>MATNQQLSIALRIQADLAEAQNALRQLTGNLQQVDRGAVQTRSELSAMGGQLDSLRAQVLGFVGAWASLSALGGLVTMVDQYGQMADRIQMVTSSTAEYEQVQARLLETASRTYRPLAEAQELYIRTADSLKSLRYTTEQALDITDSFSFLLVTNAASADRAASAIDAYSKSIQTGKVSSDAWQSIMAAMPSLVNALAESTGKSTEEIRKLGIEGSLSLRDLNEGLRKTVAANREAADNMGTSVQDALVSLNNALSAYLGELNRTYDITGSVSSALNVLAENMEVIVKLFGVAAVAGLTRYVASLTLATQAKLAAVLAARAQAAEELRTAQAQVASTAAAAANARAQAGLTVSHTQAAAAEAAHTAATQRLAAAQLAAGAAMRGMLAVIGGPAGIAMLVAGAAASFFLFRDSAQAVKSSLDDLSEPLDQVVERMGKLSEIEQDRELTRLSEQIDGLRQTAVEAAREMREVASTALYGARLDRIPSAEAQQALQPLIDASADAARGVEVDWKSVMDTLAASGAVPDSLKRKLLDMAAGQAEAGRTATELGQRHAELKARLEGSTAAINENSDALSKGSDKAAEYIQSLRLAIADLEDPSVLGKAGRRLQQFGADLNAEQSAEILRLETLKANTEKAAQAREDARRKAESSARQQASTAEQLAKSQEGYVAGLEKQARTLGLTSAEVRAYELAEKGLTGALHARAAAALAALAADEKKRQADANARTNAGLEAEYLRATGRTVDAGLLEIRTKFDAMRRDFEKAGNDAGLAWIDKLIPVAEAKVRLDDVKQQMDDLLADQQRAESSVNVQQDAGVINEMDARQRILDIHRATYEKLQQIRPILEQMARQPGEVGRAAAESLAQLDAEAARLQQTTTLLETTLRDGLTTGFTDAIKGLASGTMDLRDAITSLGEAVLNALVNMAAQNLAQSLSSGIMGLFGGGQQDTSMTTGAAAVTASAGALSTAGASLLTGAAAIQAAAASLAAANGVQGLGAAAGGAGAAGAAAGGGSWLSSIAGIFGFASGGHIKGPGTGTSDSIPILASNDEFMTRAAVVRQPGALAFLEQFNRYGMAALAGWANPVRHATGGQIGTPAPNLPAPVRAGANLPEPSKNFSTSVANSIYLHAVQDTDQMAADMWAGKGGEHFLVWLNKNRQAVKQII[3x];>MATFPGFQVPKPVEGIVAGITPNIDALELNQDISLAAVAASTWGGAYGAHQPVEVIHSTYQAVHQSALEENYYNRLWLIPTAMELGNVVSTQIRPASVWNAYFSPRTLTAIDREAADGITLSGQASPPLGFAALEERTWTVSIGTDGPPVVNARIVWRLQGEPNLVLVITGNRIIAWTFAPDWGDSIVERLSASTNILQSESAVTQRRAMRLAPRREFDANMYAVDRERQLLDMTLFGWGARIWALPIWPDIQLLHQPLAAGSLGIPCDTAGLDFRDGGLAMLRGEDAFTYEVVEVKTVTASGLDLVRPVQAAWGTGSRLYPVRTAQLTEQPTLTRLTDTAQSARVSFLVMEPSAWPELMPATTYRGRPVLEQRPDESEDLTSSYQRLLSTLDNGSAIPRVTDVAGMALPVIGHRWIGMGRAERSAFRSLVYALRGQQKPLWVPTHADDLTLVATVSQLSTALDVRNIGYARFANGRPGRRDIRIELYDGTVYHRRILTSTELDADTERVAIDAALGRLVEPTDVARICFMALCSAASDVVEIEHVTDSEGVATAALTFKGVRDDEF[3x];>MTLYMGPNTGLLINGLPGEGHYSDLIRMWRWDDFLRQPVVKGRVATLPTTGQAEGDTYIFTGSGSNQNRLARWWATGATTAIWEYMPPRLGWRVQVANETTPSGQVKTYEYSGTAWVELVGGMSDAPSDGKAYARESGAWTELGSAAKSALNVLPFMNLMPDMGRFAGTAANPLATMFTTSWTPSSFLNGWNGATVADGGKFAFDNSTNGGAGPALNARVQALLAAMGRTWTSVSRYGVEFFTAVLTAGSQTTTGSAGADGVTRYLCCSNGSKTVFNAGGWATVVMWLRVESGSAHISSAPYTTHRLWINGAVAAPGVVLPANQWVHLRFSMQSYNGYDNACPYIYASAGAQIAFACPAWFGGLVDPGIHVAPILTINGASA[9x];>MAYFTGTANNPADLLAKVRVHAESLGWVTDRASASEWLCHNADGYWSFNAGANQFQMAGNTGFDNSLAWNAQPGNSVQNNPYSSKGPTVAQLSGGPFTRYHLFATAAYLHLHVEIAAGQFRPVMIGSLNKRGVGYTGGQYVCGSFIYTPGQALTNNWSSHPFDGYHIQYSNSSCMLRLDGLDGGPSPEWLPFDYTTNVPRRVVGPGRGNYSSQYHPDVGLIDASANELNSSTTTVPCAIYAFGAQQRSRYVGEVPDFGICNMAFLAPGDPLVVGSDTWRVYPLLQRGTATDFDSTSAWVGYCFRVVE[9x];>MATEFGTAVNHADLVERLVQFLTASPDLVAAGQAYEKVFDNTIPASGTAIAVRQVTLRAPGLGGTDAIYMGIQSYGDTALDYYNLRLMGGTAFNPGAIPPGGDYWTAFANYSPRVQLLAWNQPMPYWFFANGRRFWIVVKVSTIYESAGAGFILPPCPPSQYPYPLAVVGSYRGDVATRWSDVSDRHRGISSPYERSCYLRDPAGRWLGFTVDGGAANESDYNNRTLLPLGCGRYAGSSDTVVKQLRDSFGKFPLKALQFVTRETEGRRYLGDFDGAFYVPTLNSGAEDVIVEDGVDHVVFQTAWRSGNPWLYAIRKD[9x];>[3x]MSFNSRESSLADGQPVRLYQFSRGAIRWSYNSSDRDITYQNQIFRTVPGGITDNGIICSGDPQSDQFVITAPADLDVALLYKTRSPSDAIDLVVYDMHYGDAEAAVSWVGQIGDVDWPTVDSCRITCVSEDELMDQPGLTDTYCRTCTAIVGDHRCKVNLVPYRVTLTPQSVSAWVISSGVVAGYADGWFTGGYVEWQVDGDNY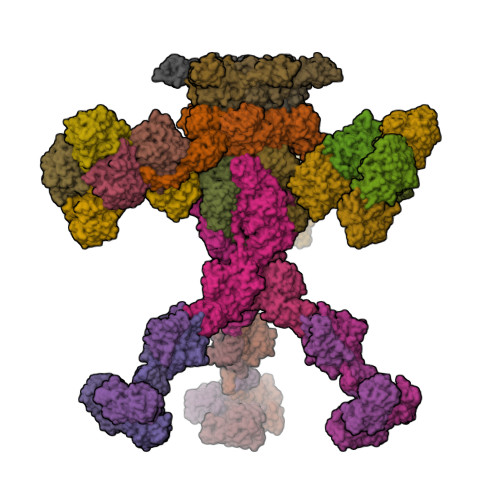DRRFIEQHAGADLHILGGTEGIPAGGQLRVYPGCDGLAQTCDDKFSNLPNFRGFNAMQGKSPFDGDQVW;>MGAKPKAQTVGWRYYFDIHFALGKKVDEVCAIRASGKTAWKGSITSNGQVRINAPELFGGDKGEGGLDGTLDVLFGEEDQGVLPRLAAMLGGLVPAFRGVTTCFYSGLVTSVNPYPKKWEILRRGGNRLWDGNPWYPEKQFVWLADGQIKAMNPAHILYLVYTGRDFRGLARTRMDEASWRAAADTLYAEGFGLCFEWTRSDSFKNFCETVKSHIGAEVYPNRQTGQISIRLLRDDYNVADLPLFDEDSGLLEITQEKTGSTSLAPSQLIVKYIDQIDGAQRQIIVNNNAVAASQGRRSSEEIEFLGVPTGELAGRVGEREMRLKTTGLKRYKGVFDRRARSLNPGQPFLIRSTPRGIPETVVRVGRIEDNFLGDGKITLTVVQDQFNLPATTGVAPPPPGWTPPDRTPRAITVRRLIEAPYRELAGVIDPANLQLLDVSASYLAALAEAPTSLSQSYTLTDRVGSSGAFVDRGTGDWCPTGLLAAELPLAAGPNVVTLTNATRLEDVTVGQAAVVDDEIVRVDAVNYASGTVTLARGCADTVPAKHLAGARVWFYDTFEAVDETVYSQGVTLQARLLTNTSEGQLAPALAATDSLTLTGRQGKPYPPGQFRINGSAYPTKVYGALSVSWAKRDRIGQADQLIDTTVGNIGPEDGATVTLQVYSGTTLKRTYAGLTSSSWSYPLAEDMADGPLQDVRLVLRSVRDGIDSWQQHDITIERHGLGFRLGEELGGVSA[3x];>[6x]MAQETYFYGQGEIDAAPIVNGVLGKWRWIQDVSAMSIQLAVEKVEHKESYSGQKALVRSFPIGKTATVNITLHSIGPDNLALTLYGKVVAKAAGSVTGEVLPADLVAGDVIRLANFGVSELVITDSASSPAPLDPQYYALRADGAYGEVQLLGLPTPAPTQPFKAAYEYAATKQVGMFTAPQPTVALRYKGINLAEGGAPVIVELYKVATDPLQELALISDGNTVAGMQISGGILLDTSKPDTGDLGRFGRIIQLG>GPSSVQLSRGDFHSIFTNKQRYDNPTGGVYQVYNTRKSDGANSNRKNLIMISDGIYHMKALLRNQAAS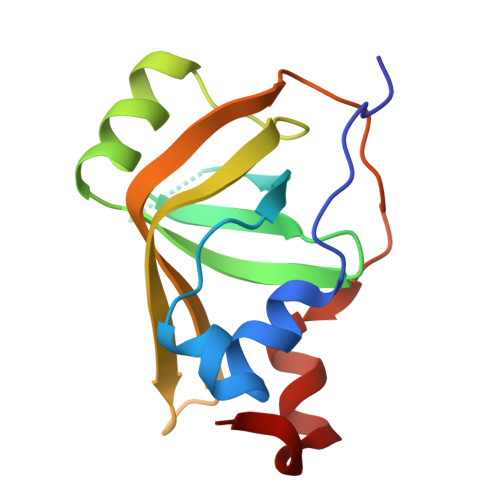KFQSMELQRGDIIRVIIAEPAIVRERKKYVLLVDDFELVQSRADMVNQTSTFLDNYFSEHPNETL[3x]> MIRLYPEQLRAQLNEGLRAAYLLLGNDPLLLQESQDAVRQVAAAQGFEEHHTFSIDPNTDWNAIFSLCQAMSLFASRQTLLLLLPENGPNAAINEQLLTLTGLLHDDLLLIVRGNKLSKAQENAAWFTALANRSVQVTCQTPEQAQLPRWVAARAKQLNLELDDAANQVLCYCYEGNLLALAQALERLSLLWPDGKLTLPRVEQAVNDAAHFTPFHWVDALLMGKSKR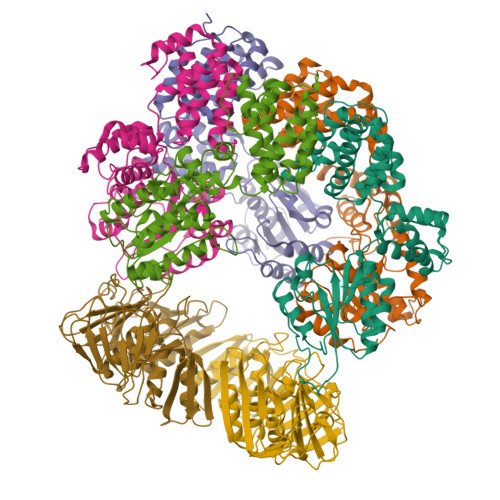ALHILQQLRLEGSEPVILLRTLQRELLLLVNLKRQSAHTPLRALFDKHRVWQNRRGMMGEALNRLSQTQLRQAVQLLTRTELTLKQDYGQSVWAELEGLSLLLCHKPLADVFIDG;>[3x]GPHMSYQVLARKWRPQTFADVVGQEHVLTALANGLSLGRIHHAYLFSGTRGVGKTSIARLLAKGLNCETGITATPCGVCDNCREIEQGRFVDLIEIDAASRTKVEDTRDLLDNVQYAPARGRFKVYLIDEVHMLSRHSFNALLKTLEEPPEHVKFLLATTDPQKLPVTILSRCLQFHLKALDVEQIRHQLEHILNEEHIAHEPRALQLLARAAEGSLRDALSLTDQAIASGDGQVSTQAVSAMLGTLDDDQALSLVEAMVEANGERVMALINEAAARGIEWEALLVEMLGLLHRIAMVQLSPAALGNDMAAIELRMRELARTIPPTDIQLYYQTLLIGRKELPYAPDRRMGVEMTLLRALAFHPRMPLPEPEVPRQ;> GPHMRWYPWLRPDFEKLVASYQAGRGHHALLIQALPGMGDDALIYALSRYLLCQQPQGHKSCGHCRGCQLMQAGTHPDYYTLAPEKGKNTLGVDAVREVTEKLNEHARLGGAKVVWVTDAALLTDAAANALLKTLEEPPAETWFFLATREPERLLATLRSRCRLHYLAPPPEQYAVTWLSREVTMSQDALLAALRLSAGSPGAALALFQGDNWQARETLCQALAYSVPSGDWYSLLAALNHEQAPARLHWLATLLMDALKRHHGAAQVTNVDVPGLVAELANHLSPSRLQAILGDVCHIREQLMSVTGINRELLITDLLLRIEHYLQPGVVLPVPHL;>[2x]GPHMKFTVEREHLLKPLQQVSGPLGGRPTLPILGNLLLQVADGTLSLTGTDLEMEMVARVALVQPHEPGATTVPARKFFDICRGLPEGAEIAVQLEGERMLVRSGRSRFSLSTLPAADFPNLDDWQSEVEFTLPQATMKRLIEATQFSMAHQDVRYYLNGMLFETEGEELRTVATDGHRLAVCSMPIGQSLPSHSVIVPRKGVIELMRMLDGGDNPLRVQIGSNNIRAHVGDFIFTSKLVDGRFPDYRRVLPKNPDKHLEAGCDLLKQAFARAAILSNEKFRGVRLYVSENQLKITANNPEQEEAEEILDVTYSGAEMEIGFNVSYVLDVLNALKCENVRMMLTDSVSSVQIEDAASQSAAYVVMPMRL> NNNRAPKEPTDPVTLIFTDIESSTALWAAHPDLMPDAVAAHHRMVRSLIGRYKCYEVKTVGDSFMIASKSPFAAVQLAQELQLCFLHHDWGTNALDDSYREFEEQRAEGECEY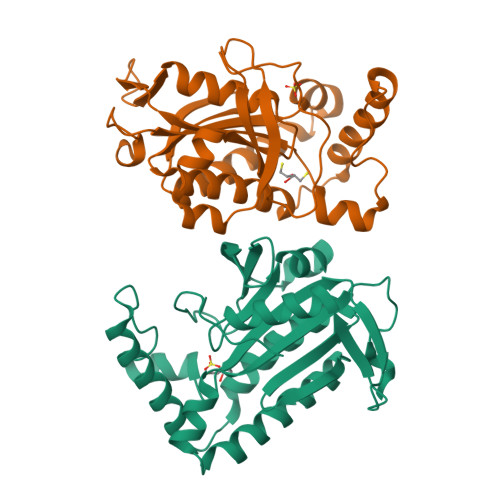TPPTAHMDPEVYSRLWNGLRVRVGIHTGLCDIRHDEVTKGYDYYGRTPNMAARTESVANGGQVLMTHAAYMSLSAEDRKQIDVTALGDVALRGVSDPVKMYQLNTVPSRNFAALRLDREYFD>[2x]MELKHSISDYTEAEFLQLVTTICDAEATSEEELDKLITHFEEMTEHPSGSDLIYWPKE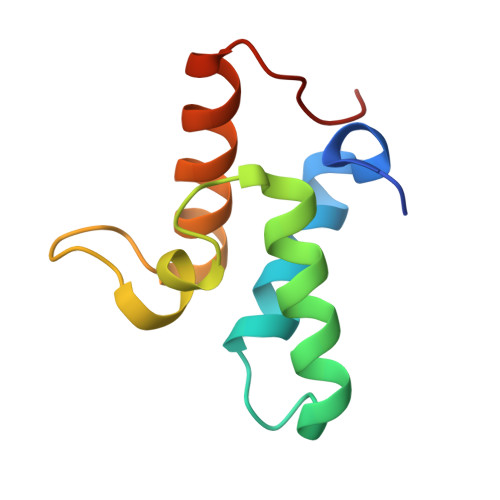GDDDSPSGIVNTVKQWRAANGKSGFKQG;>[2x]MHHHHHHSMGKRNKPGKATGKGKPVNNKWLNNAGKDLGSPVPDRIANKLRDKEFKSFDDFRKKFWEEVSKDPELSKQFSRNNNDRMKVGKAPKTRTQDVSGKRTSFELHAEKPISQNGGVYDMDNISVVTPKRHIDIHRGK>[2x]EELQKSIGHKPEPTDEEWELIKTVTEAHVATNAQGSHWKQKRKFLPEDIGQAPIVNAPEGGKVDLEAFSHFTKIITPAITRVVDFAKKLPMFCELPCEDQIILLKGCCMEIMSLRA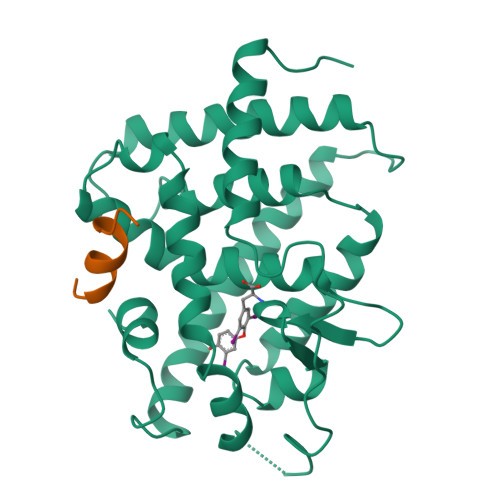AVRYDPESETLTLNGEMAVTRGQLKNGGLGVVSDAIFDLGMSLSSFNLDDTEVALLQAVLLMSSDRPGLACVERIEKYQDSFLLAFEHYINYRKHHVTHFWPKLLMKVTDLRMIGACHASRFLHMKVECPTELFPPLFLEVFED;>[2x]GHKILHRLLQDSS>[2x]MSKSKVDNQFYSVEVADSTFTVLKRYQQLKPIGSGAQG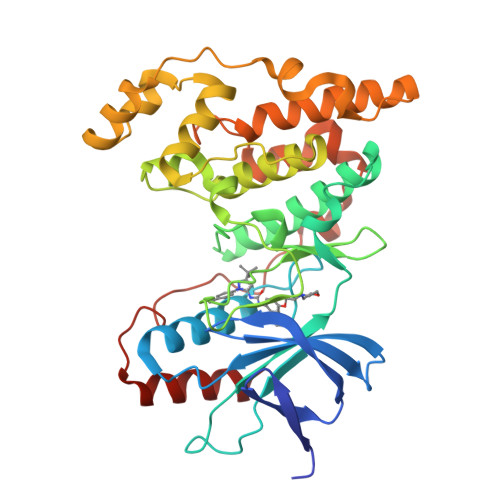IVCAAFDTVLGINVAVKKLSRPFQNQTHAKRAYRELVLLKCVNHKNIISLLNVFTPQKTLEEFQDVYLVMELMDANLCQVIHMELDHERMSYLLYQMLCGIKHLHSAGIIHRDLKPSNIVVKSDCTLKILDFGLARTACTNFMMTPYVVTRYYRAPEVILGMGYAANVDIWSVGCIMGELVKGCVIFQGTDHIDQWNKVIEQLGTPSAEFMAALQPTVRNYVENRPKYPGIKFEELFPDWIFPSESERDKIKTSQARDLLSKMLVIDPDKRISVDEALRHPYITVWYDPAEAEAPPPQIYDAQLEEREHAIEEWKELIYKEVMDWE> MASDAAAEPSSGVTHPPRYVIGYALAPKKQQSFIQPSLVAQAASRGMDLVPVDASQPLAEQGPFHLLIHKLYGDDWRAQLVAFAARHPAVPIVDPPHAIDRLHNRISMLQVVSELDHAAAQDSTFGIPSQVVVYDAAALADFGLLAALRFPLIAKPLV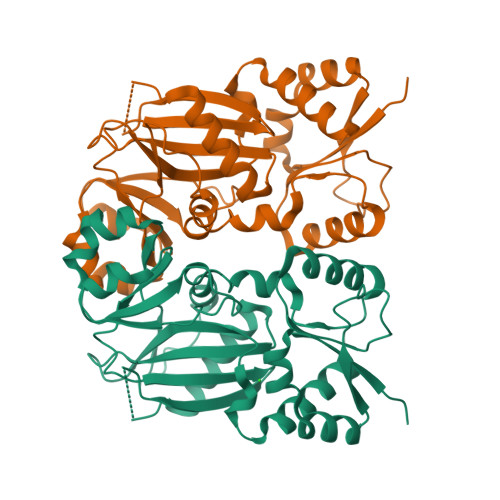ADGTAKSHKMSLVYHREGLGKLRPPLVLQEAVNAGGVIFKVYVVGGHVTCVKRRSLPDVSPEDDASAQGSVSFSQVSNLPTERTAEEYYGEKSLEDAVVPPAAFINQIAGGLRRALGLQLFNFDMIRDVRAGDRYLVIDINYFPGYAKMPGYETVLTDFFWEMVHKDGVGNQQEEKGANHVVVK> TQLEEQLHNVETVRSITMQLEM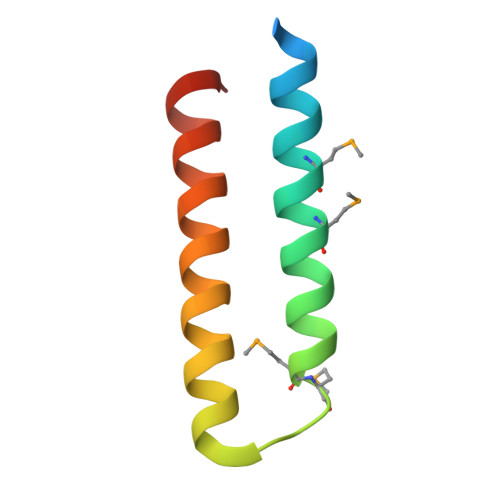ALTKLKKDMMRGGDAKQYQVWQRESKALESAIAIIHYVAGDLK>[6x]GAMEHRAKTKRNQELAEQLLKELPHETTSIANLVQRNNRDLDYNLEQLVRTLLQMEKEGTHVTESLINTLMETDTLTPKEQALIWPAYNLVRQMMHHAALHHI

The protein C is a small viral protein encoded in an overlapping frame of the P gene in the subfamily Orthoparamyxovirinae. This protein, expressed by alternative translation initiation, is a virulence factor that regulates viral transcription, replication, and production of defective interfering RNA, interferes with the host-cell innate immunity systems and supports the assembly of viral particles and budding. A previous sequence analysis revealed an architecture common to all Orthoparamyxoviridae C proteins, with a predicted N-terminal disordered moiety and a C-terminal helical moiety. We solved the crystal structure of the C-terminal part of TupV C protein at a resolution of 2.4 Å and found that it is structurally similar to Sendai virus C protein, suggesting that despite undetectable sequence conservation, these proteins are homologous.

The protein CΔ53 crystallized readily with six molecules in the asymmetric unit in the P3221 space group and diffracted at 2.4 Å resolution. The crystal structure was solved with the SAD method by soaking crystals in a platinum derivative solution, and the structure was refined to a resolution of 2.4 Å. Helix F is kinked at Pro127. The C-terminal part of helix C/D (aa 86–99), is packed onto a hairpin formed by helix E (aa 105–114) and helix F (aa 119–141). Helices D, E, and F form a small domain containing a hydrophobic core. Of note, the residues in the C-terminal part of the C/D helix (Y93, Q97, V99, (R/K)100, T101, L102, E108, and G109) that are strictly conserved among Narmoviruses are exposed to the solvent and could thus represent a recognition motif. In the first mode, two molecules of CΔ53 assembled head-to-tail, forming 14 interchain H-bonds, 2 salt bridges, and burying ~3300 Å2 of accessible surface area (PISA Complex formation Significance Score of 1.0). The chaining of asymmetric units leads to a helical assembly and to the formation of tubular structures with external diameters of ~9.0 nm and hexagonal internal cavities of 2.4–3.0 nm width. In conclusion, TupV CΔ53 is essentially monomeric in solution, in contrast with its multimeric state in the crystal.2-chloro-4-[(3S,3aS,4S)-4-hydroxy-3-methoxy-3a,4,5,6-tetrahydro-3H-pyrrolo[1,2-b]pyrazol-2-yl]-3-methylbenzonitrile 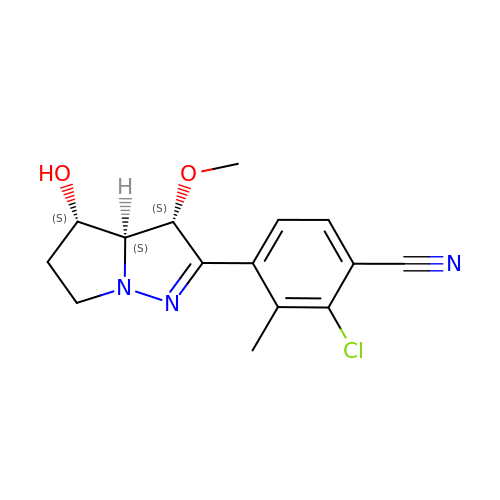| C15 H16 Cl N3 O2 | RJZJEPYCJHLWQR-TUKIKUTGSA-N> TDTIKF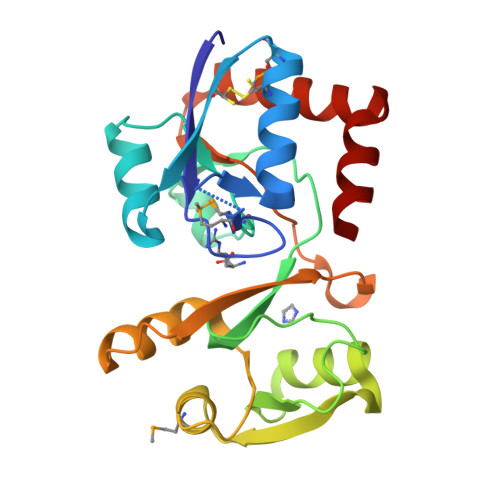ATEATYPPYVYMGPSGQVEGFGADIVKAVCKQMQAVCTISNQPWDSLIPSLKLGKFDALFGGMNITTARQKEVDFTDPYYTNSVSFIADKNTPLTLSKQGLKGKIIGVQGGTTFDSYLQDSFGNSITIQRYPSEEDALMDLTSGRVDAVVGDTPLIKQWLKQNGRREYVLIGKPVNDPNYFGKGVGIAVKKGNQALLLKLNKALAAIKANGVYAAIVQKYF> KKAVINGEQIRSISDLHQTLKKELALPEYYGENLDALWDALTGWVEYPLVLEWRQFEQSKQLTEN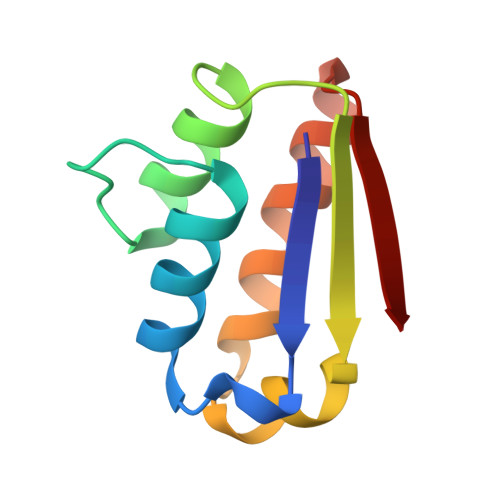GAESVLQVFREAKAEGADITIILS We characterized biochemically and structurally the opit5_10225 gene product, and show that the enzyme, Op5Man5, is an exo-β-1,4-mannosidase [EC 3.2.1.25] that is highly specific for β-1,4-mannosidic bonds in mannooligosaccharides and ivory nut mannan. Op5Man5 features a 200-kDa large homotrimer composed of three modular monomers. The modular monomer structure contains an N-terminal catalytic (β/α)8 (TIM) barrel that belongs to clan GH-A with a sequence placed in the GH5 family of retaining glycoside hydrolases (domain A; residues 2–364). The A-domain is followed by a Rossmann-like β-sandwich domain (domain B; residues 367–586).

Op5Man5 crystallized in space group P212121 with one homotrimer per asymmetric unit and diffracted to 2.2 Å resolution. Crystals of Op5Man5 grew from a solution containing phosphorus citrate (pH 4.2), 30% (v/v) ethanol, 5% (w/v) polyethylene glycol 1000, and were subjected to soaking with 1 mM UO2(NO3)2. The partial model was then used to phase the 2.2-Å X-ray diffraction data using molecular replacement to determine the crystal structure of Op5Man5. As expected for an exo-acting β-mannosidase, the active site in Op5Man5 is located in a pocket with the two catalytic glutamate residues (Glu156 and Glu281) buried roughly 10 Å below the surface of domain A. All three active sites are accessed from the central void of the homotrimer. Two loop regions in Op5Man5 (residues 103–108 and 320–339) cooperate to form a steric block that closes off the active site to form a pocket. The steric block has been assigned a structural role in converting a GH5-type endo-mannanase into an exo-acting mannosidase (Zhou et al., 2014, Dias et al., 2004). There are no salt bridges formed between individual monomers, and trimer stabilization is partly provided through 17 hydrogen bonds between the B-domain and the A-domain of a neighboring monomer. There are no direct interactions between B domains of individual monomers in the trimer. Two regions in Op5Man5 map have weak, unresolved electron density, and were therefore not modeled: a flexible region in domain A between β5 and β6, including the region expected to form α5 (residues 213–221); and the linker region that connects domains A and B (residues 368–381). The missing regions are located at the surface, on the side of the TIM barrel opposite to the active-site entrance, and neither is therefore expected to influence substrate binding or catalysis.

>[3x]MTIDSSGYFRDAAGARFIPVGANYWPASCGVEMWQAWPEDEIFSDLDLMASLGFNTVRFFVRWPDFEPRPGEYDATMLSRLLRLLDACGERGLRPQPSLFVGWMSGGIFWPPWKSDTQNLFSDPVMIERGAAYARTITTHLKPFATHLCGIDLGNELDALPDCSAATPAQVHEWCRRMTGAIREVLPEALILSGCDHQQVIADTGWRLGGSSPCYSAGGTPAPRMVPNPAQPGIDVLTMHGYPVPNWHPVQGSGLADPLTRSLLPFYVKCARAFGPVLLQEFGTILTSRAAAPHTDAYLRAILPACREAGANGYLWWCFKDIPAPLHPYIKNNFESELGLVDIEGRVKKGLEYFVEFARAETQRALKVLTACEQLDHSAEDAPTVHLYWPRHYYHRNNHRNPGNEPRETSRRLILAHHLLQSAEEHVGIVRGDQPLPSPSEVERIIITGVFTGLDEIKELHSWVEQGGQLLWHAPDPVNWAQAMSRLVGAEIADYRAATPAITATDEGPYEFTCFLRGMRVRIEPRGAQILMTDNEGSPLVLRHRVGAGCVTSVLADVEASFLSQWPDRQTQEASWSAWYAALLTKDQSEGVARAHHHHHH> MRPPQFTRAQWFAIQHIDSDSSPSSSSRYCTIAMRAINNYRWRCKPVNTFVHEPLVDVQNVCFQEKV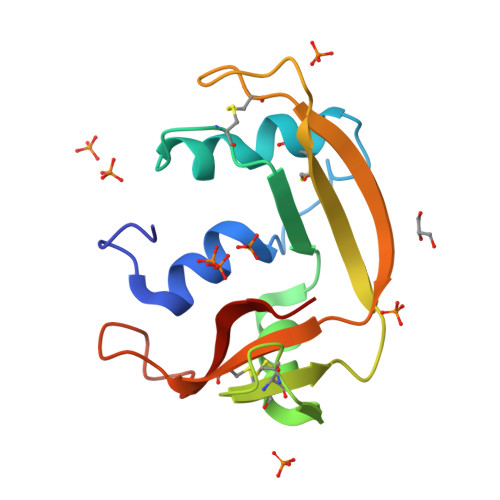TCKNGQGNCYRSRFRMHITDCRLTNGSRYPNCRYRTRPGRRHIIVACENRDPRDSPRYPYVPVHFDASV>[6x]AGITGTWYNQLGSTFIVTAGADGALTGTYESAVGNAESRYVLTGRYDSAPATDGSGTALGWTVAWKNNYRNAHSATTWSGQYVGGAEARINTQWLLTSGTTEANAWKST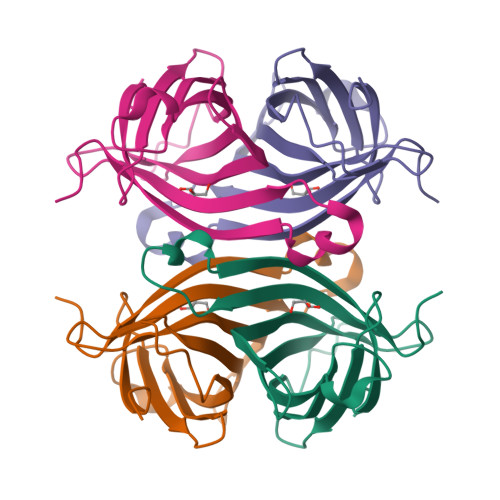LVGHDTFTKVKPSAAS Desmosomes are intercellular junctions that confer structural integrity to tissues by linking the intermediate filament cytoskeletons of adjacent cells. The cytosolic armadillo proteins plakoglobin and plakophilins interact with desmosomal cadherins and with desmoplakin (DP), a member of the plakin family of cytolinkers. The 912 amino acid C-terminal region (DPCT) binds to intermediate filaments (IFs), including keratins, vimentin and desmin. DPCT contains three plakin repeat domains (PRDs), designated PRD-A, PRD-B, and PRD-C, which share ~30% sequence identity with each other.

We determined the crystal structure of PRD-AB consisting of residues 1960–2248 at 2.6 Å resolution. There is one copy in the asymmetric unit, consistent with size exclusion chromatography indicating that it is a monomer in solution. The two domains are arranged in a “beads on a string” manner to form an elongated structure with approximate overall molecular dimensions 38 Å × 42 Å × 108 Å. Domain B is related to domain A by a 54 Å translation along a common long axis of the two domains, and a rotation of 29°. The two domains are connected by a 4 amino acid linker (residues 2204–2207) but do not form any direct contacts (interatomic distance < 4 Å) with one another. In fact, the amino acids comprising the linker have higher temperature factors than nearby residues and do not form direct contacts with either domain. Although the overall structure of PRD-A is similar to that of PRD-B, it has a markedly different surface charge profile. Whereas domains B and C are acidic proteins (calculated pIs ~ 4.7 and 5.8), domain A is highly basic (pI ~9.0). Superposition of the three domains of DPCT shows that their overall structures are very similar. The principal difference among PRDs A, B and C is the presence of an additional N-terminal PR-like motif in PRD-A and –B that protrudes from the globular domain formed by the 4.5 PRs (grey in Fig 2). The envelope clearly showed that there are two domains but, in contrast to linear arrangement of domains A and B in the crystal structure, the SAXS envelope revealed a bent conformation.

> GAMGSTVDTSKLVFDGLRKKVTAMQLYECQLIDKTTLDKLLKGKKSVEEVASEIQPFLRGAGSIAGASASPKEKYSLVEAKRKKLISPESTVMLLEAQAATGGIIDPHRNEKLTVDSAIARDLIDFDDRQQIYAAEKAITGFDDPFSGKTVSVSEAIKKNLIDRETGMRLLEAQIASGGVVDPVNSVFLPKDVALARGLIDRDLYRSLNDPRDSQKNFVDPVTKKKVSYVQLKERCRIEPHTGLLLLSVQKRSMSFQGIRQPVTVTELVDSGILRPSTVNELESGQISYDEVGERIKDFLQGSSCIAGIYNETTKQKLGIYEAMKIGLVRPGTALELLEAQAATGFIVDPVSNLRLPVEEAYKRGLVGIEFKEKLLSAERAVTGYNDPETGNIISLFQAMNKELIEKGHGIRLLEAQIATGGIIDPKESHRLPVDIAYKRGYFNEELSEILSDPSDDTKGFFDPNTEENLTYLQLKERCIKDEETGLCLLPLKE The PH domain-containing protein Slm1 from budding yeast Saccharomyces cerevisiae is required for actin cytoskeleton polarization and cell growth. The PH domain-containing protein Slm1 from S. cerevisiae is a component of the target of rapamycin complex 2 (TORC2) signaling pathway. We have previously reported that in vitro, the Slm1-PH domain (Slm1-PH) interacts with liposomes containing PtdIns(4,5)P2 and DHS-1P cooperatively. The core of each monomer consists of seven antiparallel β-strands with a C-terminal amphipathic α-helix connected via a long and flexible loop.

The results presented here include: (i) the apo structure of Slm1-PH that we resolved at 1.76 Å resolution; (ii) one structure with phosphoserine at 1.68 Å resolution; and (iii) two structures of Slm1-PH in complex with Ins(4)P at 1.4 and 1.8 Å resolution. Electron densities corresponding to the Ins(4)P molecules were visible between the β1-β2 and β5-β6 loop regions (difference density maps). For the two structures determined in complex with Ins(4)P, the positions of the inositol ring overlap. In both cases, the oxygen atoms of the inositol ring contact the β1-β2 region through the hydroxyl group of Tyr485 (hydrogen bond length  = 2.8 Å) and the NH2 group of Arg478 (hydrogen bond length  = 2.5 Å), and the β5-β6 loop through the ε-amino group of Lys542 (hydrogen bond length  = 2.7 Å). In addition, we observed a contact with the ε-amino group of Lys562 (hydrogen bond length  = 3.2 Å) from the β6-β7 strand. Interestingly, the two structures differ with respect to the orientation of the phosphate at position 4 (P4), which contacts either the β1-β2 loop or turns 180° and contacts the β5-β6 loop. In the first case, the main-chain nitrogen of Tyr485 and the carbonyl oxygen of Ser484 (hydrogen bond lengths  = 3.0 and 3.1 Å, respectively) of the β1-β2 loop region interact with P4, whereas in the other structure the main-chain nitrogen atom of Ser539 of the β5-β6 loop forms hydrogen bonds of 2.6 Å with the oxygen atom of P4. In the non-canonical binding site there are four residues that are consistently involved in ligand binding: Arg478, Tyr485, Lys542 and Lys562. The non-canonical binding site is shallow, large and solvent-exposed, and so the phosphate position of Ins(4)P in one of the structures was seen on the opposite side of the molecule. * Crystals of the same protein-ligand complex were obtained in different crystallization conditions.

>[4x]DHPFTEIKSGFLERRSKFLKSYSKGYYVLTPNFLHEFKTADRKKDLVPVMSLALSECTVTEHSRKNSTSSPNSTGSDAKFVLHAKQNGIIRRGHNWVFKADSYESMMSWFDNLKILTSTS>PMFIVNTNVPRASVPDGFLSELTQQLAQATGKPPQYIAVHVVPDQLMAFGGSSEPCALCSLHSIGAIGGAQNRSYSKLLCGLLAERLRISPD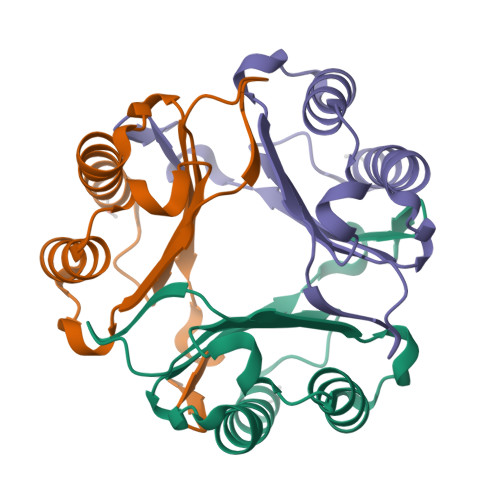RVYINYYDMNAANVGWNNSTFA[3x]>GTGGTGGTGGTG[2x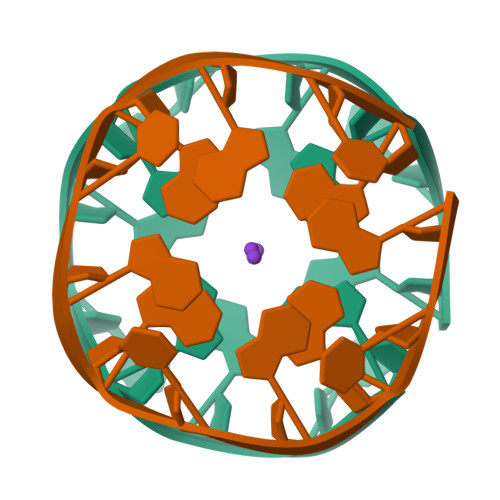]> 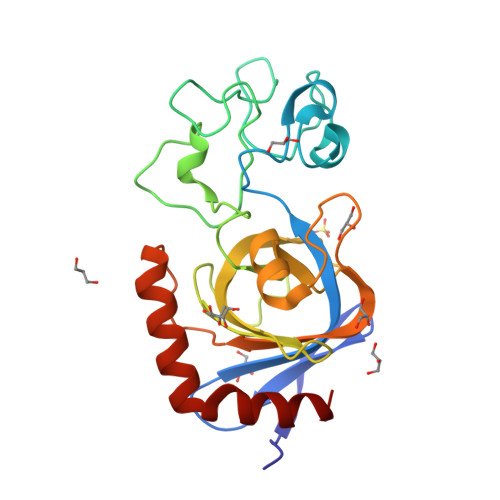HMSELSEIDSVAGVTIYSVDGEPKSFVYKAGFAIDADGAPNAYAPNNGGTDFTANGGDDQGGDWWGGPVDAEGYPIKQKIFDPFPGYYVSATAHFNPAYSEDSPYRYIDSNSIPFIVLPGNHSNGAKLGDVALVYNEKTGDNCYAIYGNVGPSSKIGEGSVRLAQALKIDDNPKAGGTESRIVVTLVFPGSVGKWETPKRWFSHANQLTKAWGGLSRLKTLSDQL>[2x]GEVINQPMMMAAQQLHREATKWSSKGNDIIAAAKRMALLMAEMSRLVRGGSGTKRALIQCAKD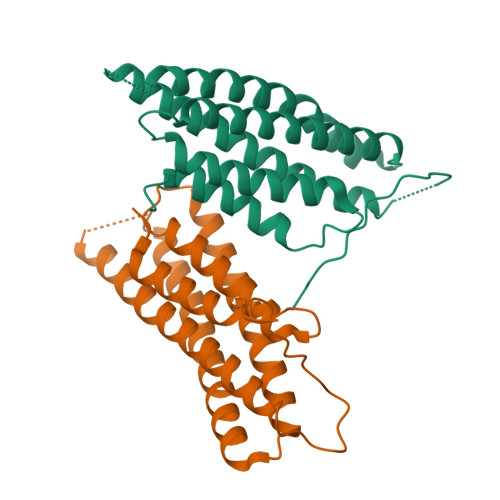IAKASDEVTRLAKEVAKQCTDKRIRTNLLQVCERIPTISTQLKILSTVKATMLGRTNISDEESEQATEMLVHNAQNLMQSVKETVREAEAASIKIRTDAGFTLRWVRKTPWYQ>[2x]MSKTQEFRPLTLPPKLSLSDFNEFIQDIIRIVGSENVEVISSKDQIVDGSYMKPTHTHDPHHVMDQDYFLASAIVAPRNVADVQSIVGLANKFSFPLWPISIGRNSGYGGAAPRVSGSVVLDMGKNMNRVLEVNVEGAYCVVEPGVTYHDLHNYLEANNLRDKLWLDVPSLGGGSVLGNAVERGVGYTPYGDHWMMHSGMEVVLANGELLRTGMGALPDPKRPETMGLKPEDQPWSKIAHLFPYGFGPYIDGLFSQSNMGIVTKIGIWLMPNPGGYQSYLITLPKDGDLK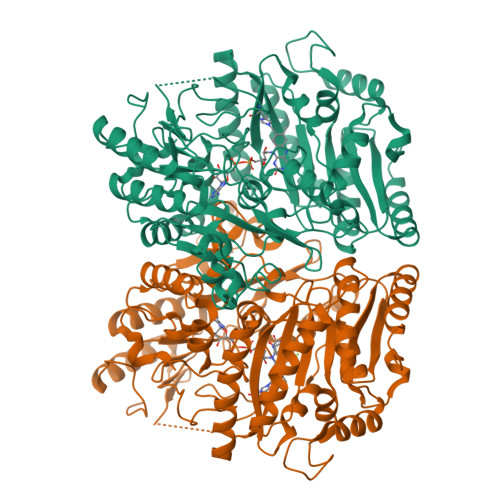QAVDIIRPLRLGMALQNVPTIRHILLDAAVLGDKRSYSSRTEPLSDEELDKIAKQLNLGRWNFYGALYGPEPIRRVLWETIKDAFSAIPGVKFYFPEDTPENSVLRVRDKTMQGIPTYDELKWIDWLPNGAHLFFSPIAKVSGEDAMMQYAVTKKRCQEAGLDFIGEFTVGMREMHHIVCIVFNKKDLIQKRKVQWLMRTLIDDCAANGWGEYRTHLAFMDQIMETYNWNNSSFLRFNEVLKNAVDPNGIIAPGKSGVWPSQYSHVTWKL>MSLELPFSNQSIIPAAHNQKDMEKILELDLTYMVMLETHVAQLKALVKYAQAGGKKVLLHADLVNGLKNDDYAIDFLCTEICPDGIISTRGNAIMKAKQHKMLAIQRLFMIDSSAYNKGVALIQKVQPDCIELLPGIIPEQVQKMTQKLHIPVIAGGLIETSEQVNQVIASGAIAVTTSNKHLWEGHHH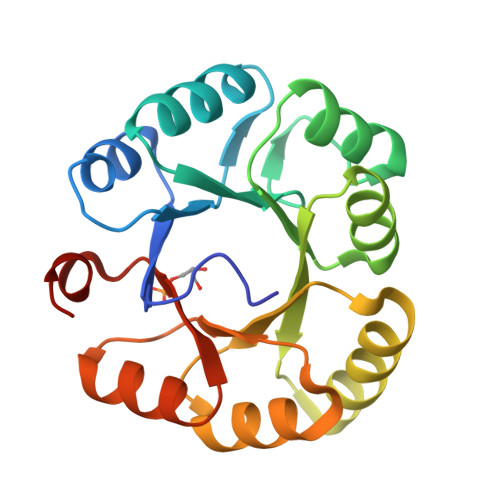HHH[8x]> MGSSHHHHHHSQDPMNDCDEKNLTNHFTFGDDLL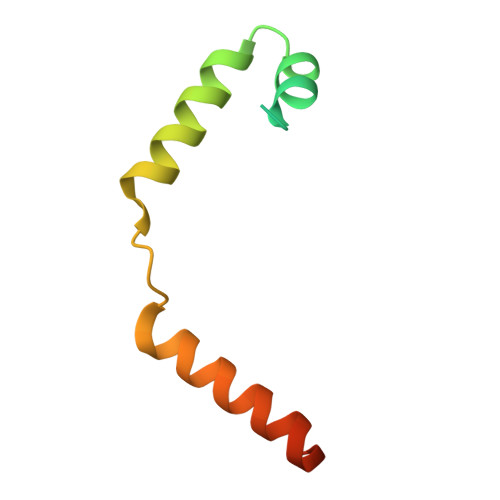GVNSEIARKLRQFYLEIQEEALPARLLELLERLEQAERFGLNNAEKV PHOSPHONOPYRUVATE 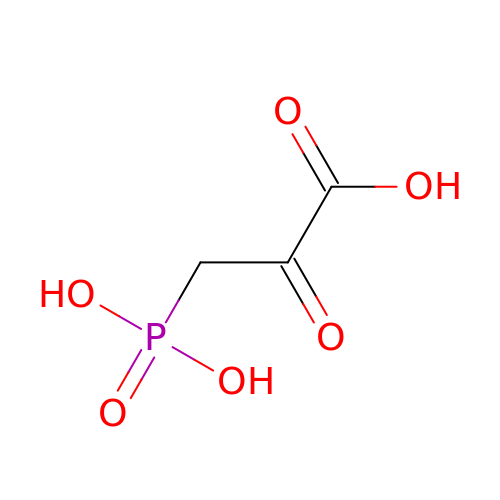| C3 H5 O6 P | CHDDAVCOAOFSLD-UHFFFAOYSA-N>SVVELGKMIIQETGKSPFPSYTSYGCFCGGGERGPPLDATDRCCLAHSCCYDTLPDCSPKTDRY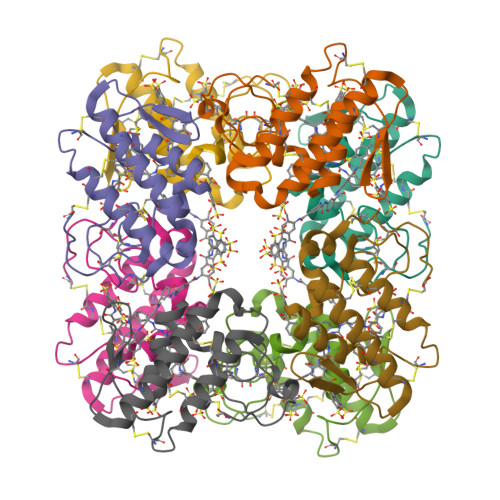KYKRENGEIICENSTSCKKRICECDKAVAVCLRKNLNTYNKKYTYYPNFWCKGDIEKC[8x]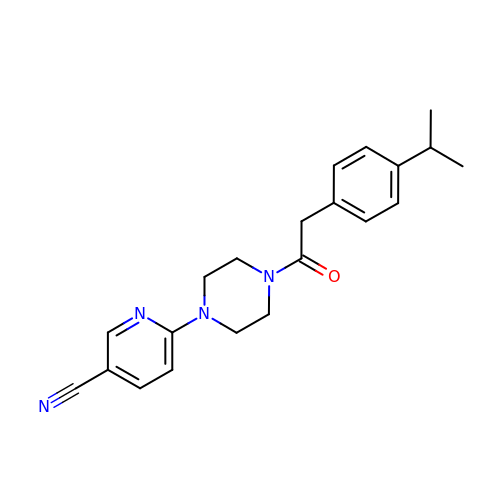6-(4-{[4-(propan-2-yl)phenyl]acetyl}piperazin-1-yl)pyridine-3-carbonitrile | C21 H24 N4 O | KJRSRHAWEMYUSP-UHFFFAOYSA-N>[2x]PHEELQYLRQLREILCRGSDRLDRTGIGTLSLFGMQARYSLRDHFPLLTTKRVFWRGVVQELLWFLKGSTDSRELSRTGVKIWDKNGSREFLAGRGLAHRREGDLGPVYGFQWRHFGAAYVDADADYTGQGFDQLSYIVDLIKNNPHDRRIIMCAWNPADLSLMALPPCHLLCQFYVADGELSCQLYQRSGDMGLG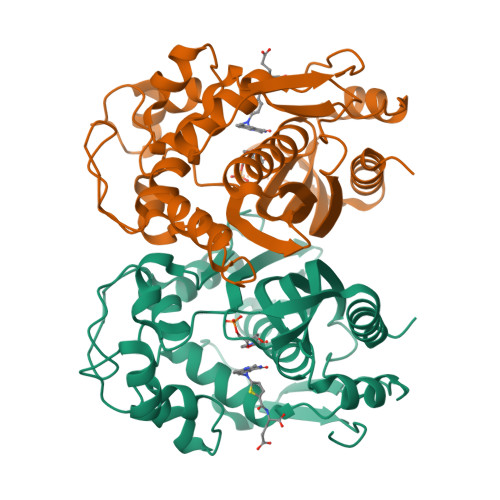VPFNIASYSLLTYMLAHVTGLRPGEFIHTLGDAHIYKTHIEPLRLQLTRTPRPFPRLEILRSVSSMEEFTPDDFRLVDYCPHPTIRM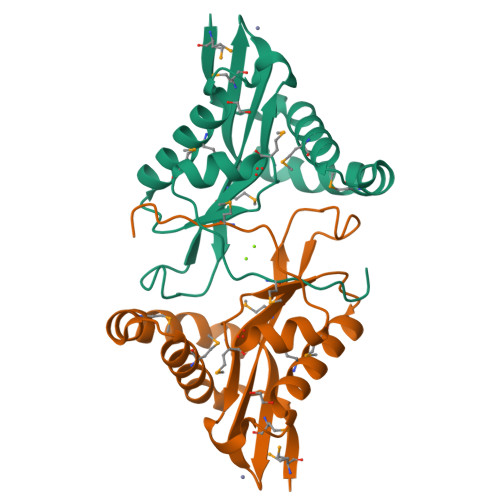> GMECRPLCIDDLELVCRHREAMFREAGRDALTLAAMQDPFRDWLLPRLADGSYFGWVMEEGGAPLAGIGLMVIEWPPHPSHPLQDKRGYILNLYVDPSHRERGIGQALMNRAEAEFAERGIAFAVLHATEMGQPLYARMGWSPTTEMSKPIAG> YLTERDTKMIMEILDNPPAPNEKLLAAAFALPD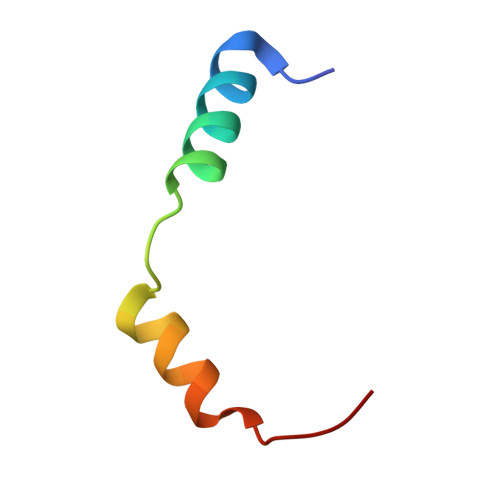MKK> SHMMRNRSVRNIVWDIGEKLSDYEKVKEIVNNEKNYINFEGNFLNPFNELSLSHGIPALCVLYGELNEQYPEQGWDVIGHEYMKRMGEYIEEKGITSLSMFSGVSGIGLSAVCLSNNRSRYGNFISSMNSFIEENIPGFIEILRNKESLNMSDYDVIEGVCGIANYCMLFPNNEEMKQALRLIVGYIIELCKDKTINGLVLPGWYISAENQFSKVDQKLWPEGCFNIGLSHGVPGMLLVLCNSTKCGIHLEDQDDSINKLVDFLIKFHISNDKENYWGSHISLEEYREGKVNSTNSRDAWCYGTPGAAYSVLIAGKYLNNMEYIDEAVNAMKGAINRLRDIYSPTFCHGFSGIAYISNRFYEVTKQQDFKKAAIDLTDKILELYDEKAPFGFYNMEKSEEGMDYLDYIGIIDGVTGIILTLLAIENGKKTPWDCAFSLQEVAAAHHAAA

In this study, we focused on class I cyclases (LanC), which catalyze the nucleophilic attack of a thiol group (cysteine) towards the previously dehydrated amino acids Dha or Dhb yielding Lan or Me-Lan rings, respectively. Although, the lanthionine ring formation can occur at basic pH values (pH > 7.5) without LanC, the enzyme is still necessary for the correct ring topology by facilitating the regio-and stereoselectivity of the catalyzed reaction. In this study, we focused on a lanthipeptide called maddinglicin (MadA) found in the genome of Clostridium sp. maddingley, which was isolated from a coal-seam formation water sample in Maddingley (Australia) in 2013. Here, we determined the structure of a class I cyclase (MadC), involved in the modification of maddinglicin (MadA) via X-ray crystallography at a resolution of 1.7 Å, revealing new insights about the structural composition of the catalytical site.

The crystal structure of MadC from C. maddingley revealed an α,α-toroid structure consisting of seven helices each (in total 14 helices), a catalytical zinc ion and a SH2-like domain as already described for NisC (Li et al., 2006). The SH2-like domain is assumed to bind the leader region of maddinglicin and has high resemblance to eukaryotic peptide-binding domains. The zinc ion is coordinated by two cysteines (Cys298; Cys344), one histidine (His345) and one water molecule. Beside the conservation of the coordinating residues also the histidine (His228) and arginine (Arg294) residues, which are proposed to be essential for the acid/base chemistry are conserved. Interestingly, an extended β-sheet (aa 391–402) is present at the opposite site of the SH2-like domain, which was so far not observed in class I LanCs (highlighted in cyan). The zinc ion is located in the center between these two structural features. Unfortunately, the amino acids from position 26 to 45 could not be modelled due to poor electron density in this region. Interestingly, the NisC structure also revealed poor electron density (aa position 28 to 32) in the same region, which leads to the assumption that this region represents a highly flexible part in LanC’s. The missing electron density for these amino acids could be explained by a high flexibility in the ligand-free (apo state) which could be shifted to a more ordered conformation after binding of a substrate. For the determination of the oligomeric state, SEC coupled to multi angle light scattering (SEC-MALS) was used and revealed that MadC is a monomer in solution with a molecular weight of 49.44 kDa ± 0.05 kDa, which is close to the theoretically calculated molecular weight of 49.71 kDa based on the sequence.> GSHMSHLDNTMAIRLLPLPVRAQLCAHLDALDVWQQLATAVKLYPDQVEQISSQKQRGRSASNEFLNIWGGQYNHTVQ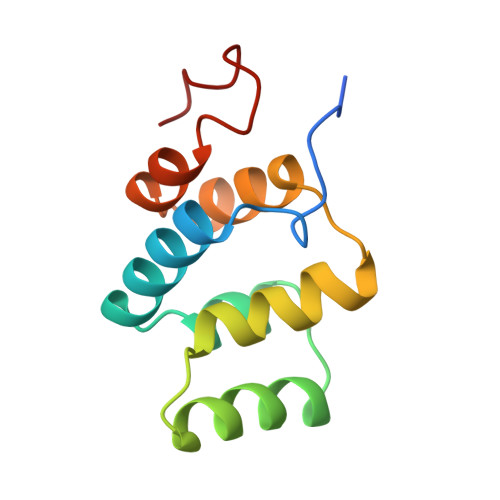TLFALFKKLKLHNAMRLIKDYVSEDLHKYI> SLTE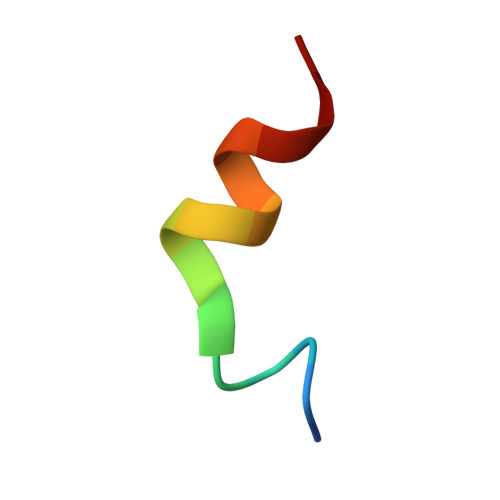RHKILHRLLQE>[3x]GPAMLPISMSDEGDSFLVKDSLGENKIPKNPSKVVILDLGILDTFDALKLNDKVVGVPAKNLPKYLQQFKNKPSVGGVQQVDFEAINALKPDLIIISGRQSKFYDKLKEIAPTLFVGLDNANFLSSFENNVLSVAKLYGLEKEALEKISDIKNEIEKAKSIVDEDKKALIILTNSNKISAFGPQSRFGIIHDVLGINAVDENIKVGTLGKSINSEFILEKNPDYIFVVDR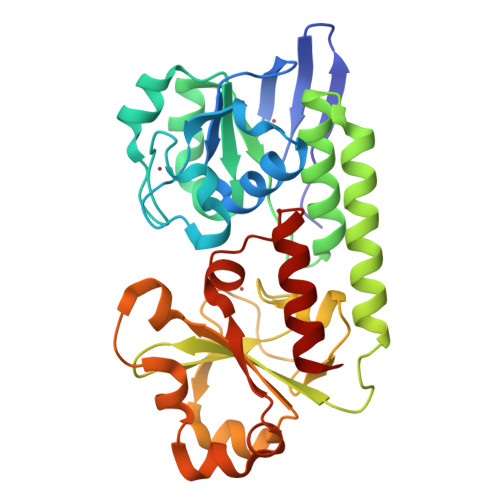NVILGNKERAQGILDNALVAKTKAAQNKKIIYLDPEYWYLASGNGLESLKTMILEIKNAVK> MRGSHHHHHHGSREGRFVPGTPRHGFVEGTEGALPKQADVVVVGAGILGIMTAINLVERGLSVVIVEKGNIAGEQSSRFYGQAISYKMPDETFLLHHLGKHRWREMNAKVGIDTTYRTQGRVEVPLDEEDLVNVRKWIDERSKNVGSDIPFKTRIIEGAELNQRLRGATTDWKIAGFEEDSGSFDPEVATFVMAEYAKKMGVRIYTQCAARGLETQAGVISDVVTEKGAIKTSQVVVAGGVWSRLFMQNLNVDVPTLPAYQSQQLISGSPTAPGGNVALPGGIFFREQADGTYATSPRVIVAPVVKESGGSSTALPDLPELNASLEKLKAEFPAFKESKLIDQWSGAMAIAPDEN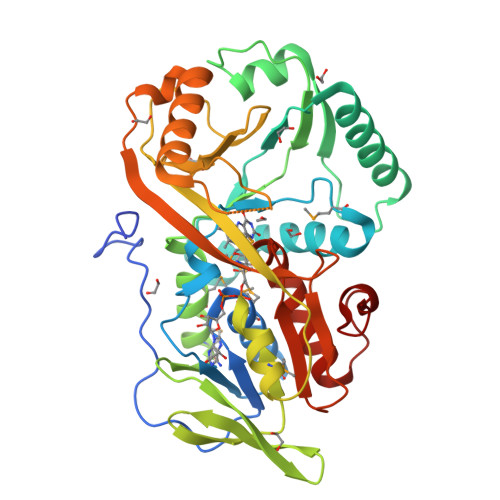PIISEVKEYPGLVINTATGWGMTESPVSAELTADLLLGKKPVLDPKPFSLYRF> SDQTWVQCDACLKWRKLPDGMDQLPEKWYCSNNPDPQFRNCE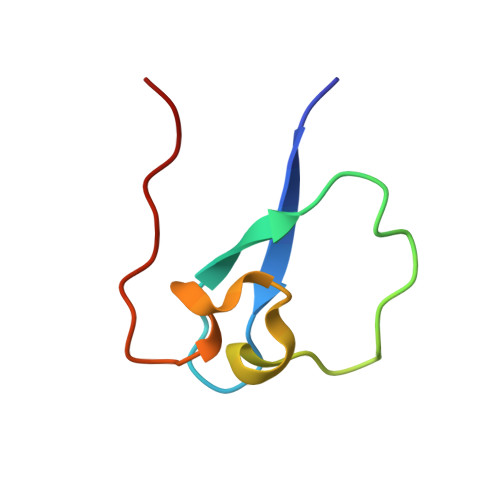VPEEPEDE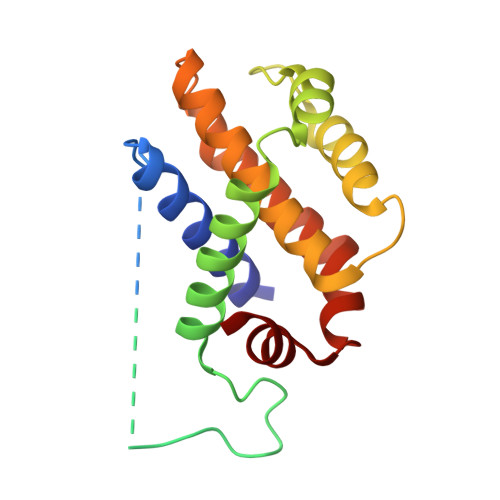>[2x]MSQSNRELVVDFLSYKLSQKGYSWSQFSDVEENRTEAPEETEAERETPSAINGNPSWHLADSPAVNGATGHSSSLDAREVIPMAAVKQALREAGDEFELRYRRAFSDLTSQLHITPGTAYQSFEQVVNELFRDGVNWGAIVAFFSFGGALCVESVDKEMQVLVSRIASWMATYLNDHLEPWIQENGGWDTFVDLYG>[2x]MITAQAVLYTQHGEPKDVLFTQSFEIDDDNLAPNEVIVKTLGSPINPSDINQIQGV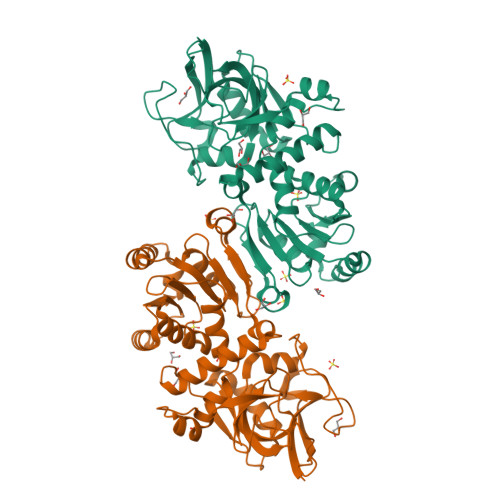YPSKPAKTTGFGTAEPAAPCGNEGLFEVIKVGSNVSSLEAGDWVIPSHVNFGTWRTHALGNDDDFIKLPNPAQSKANGKPNGLTINQGATISVNPLTAYLMLTHYVKLTPGKDWFIQNGGTSAVGKYASQIGKLLNFNSISVIRDRPNLDEVVASLKELGATQVITEDQNNSKEFGPTIKEWIKQSGGEAKLALNCVGGKSSTGIARKLNNNGLMLTYGGMSFQPVTIPTSLYIFKNFTSAGFWVTELLKNNKELKTSTLNQIIAWYEEGKLTDAKSIETLYDGTKPLHELYQDGVANSKDGKQLITY> SPQPLEQIKLSESQLSGRVGMIEMDLASGRTLTAWRADERFPMMSTFKVVLCGAVLARVDAGDEQLERKIHYRQQDLVKYSPVS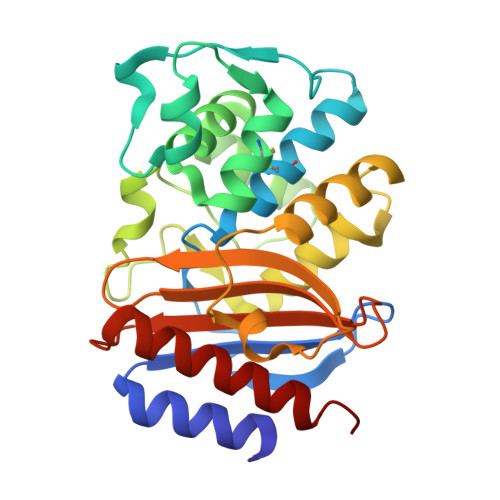EKHLADGMTVGELCAAAITMSDNSAANLLLATVGGPAGLTAFLRQIGDNVTRLDRWETELNEALPGDARDTTTPASMAATLRKLLTSQRLSARSQRQLLQWMVDDRVAGPLIRSVLPAGWFIADKTGAGERGARGIVALLGPNNKAERIVVIYLRDTPASMAERNQQIAGIGAALIEHWQR(2S)-PYRROLIDIN-2-YLMETHYLAMINE | C5 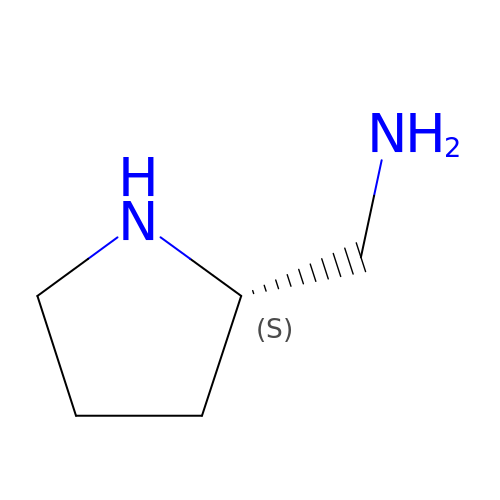H12 N2 | AUKXFNABVHIUAC-YFKPBYRVSA-N TRPM8 is a multimodal sensor of innocuous-to-noxious cold that is activated by several factors, such as temperature, cooling agents (e.g., menthol and icilin), voltage, pressure, and osmolality. TRPM8 is a non-selective cation channel permeable to both monovalent and divalent cations that is activated by multiple factors, such as temperature, voltage, pressure, and changes in osmolality. TRPM8 has attracted great interest because of the therapeutic applications of its modulators that can be utilized for several pathological conditions, including neuropathic pain, irritable bowel syndrome, oropharyngeal dysphagia, chronic cough, and hypertension. At 2.7 Å resolution, it is one of the two highest-resolution structures of any TRPM8 protein that is currently available. Overall, human TRPM8 adopts a characteristic homotetrameric arrangement and is very similar to previously described TRPM8 structures.

We determined a cryo-EM structure of apo HsTRPM8 that was solubilized with lauryl maltose neopentyl glycol (LMNG) and cholesteryl hemisuccinate (CHS). By combining a high-resolution global map with focused refinement maps of N-terminal domains, we were able to build an atomic model of human TRPM8 (HsTRPM8) that comprises residues 43–1104. The pore is composed of helices S5 and S6 connected with a pore helix (PH). The lower gate of the channel is formed by hydrophobic side chains of M978 and F979 (both shown in Fig. 2a as sticks) that close the pore. In contrast, in our reconstruction, only the first two amino acids from the selectivity filter (F912 and G913) are resolved. The conformation of the pore in our structure is similar to the closed C0 MmTRPM812. In our structure, the S4-S5 linker is parallel to the S5 helix, and the S4 helix is fully α-helical. The quality of our EM map in this region allowed us to unambiguously assign them to two CHS molecules and a phospholipid with one monounsaturated fatty acid which we modeled as phosphatidylcholine (POPC). In summary, additional densities visible in our HsTRPM8 (and other published structures) can be interpreted as compounds copurifying with the protein (PE/POPC, Na+) or used for its solubilization (CHS), but we cannot be sure about their identity and source, and thus interpret their physiological relevance. Importantly, we did not observe any density in the putative Ca2+-binding pocket between the S2 and S3 helices that could be assigned to the divalent ion, which further confirms that our structure is not in the desensitized state. To improve the quality of the reconstruction of this region we performed its focused refinement, followed by C4 symmetry expansion and subtraction of the signal from the rest of the TRPM8 molecule.

>[4x]SNSFRAARLSMRNRRNDTLDSTRTLYSSASRSTDLSYSESDLVNFIQANFKKRECVFFTKDSKATENVCKCGYAQSQHMEGTQINQSEKWNYKKHTKEFPTDAFGDIQFETLGKKGKYIRLSCDTDAEILYELLTQHWHLKTPNLVISVTGGAKNFALKPRMRKIFSRLIYIAQSKGAWILTGGTHYGLMKYIGEVVRDNTISRSSEENIVAIGIAAWGMVSNRDTLIRNCDAEGYFLAQYLMDDFTRDPLYILDNNHTHLLLVDNGCHGHPTVEAKLRNQLEKYISERTIQDSNYGGKIPIVCFAQGGGKETLKAINTSIKNKIPCVVVEGSGQIADVIASLVEVEDALTSSAVKEKLVRFLPRTVSRLPEEETESWIKWLKEILECSHLLTVIKMEEAGDEIVSNAISYALYKAFSTSEQDKDNWNGQLKLLLEWNQLDLANDEIFTNDRRWESADLQEVMFTALIKDRPKFVRLFLENGLNLRKFLTHDVLTELFSNHFSTLVYRNLQIAKNSYNDALLTFVWKLVANFRRGFRKEDRNGRDEMDIELHDVSPITRHPLQALFIWAILQNKKELSKVIWEQTRGCTLAALGASKLLKTLAKVKNDINAAGESEELANEYETRAVELFTECYSSDEDLAEQLLVYSCEAWGGSNCLELAVEATDQHFIAQPGVQNFLSKQWYGEISRDTKNWKIILCLFIIPLVGCGFVSFRKKPVDKHKKLLWYYVAFFTSPFVVFSWNVVFYIAFLLLFAYVLLMDFHSVPHPPELVLYSLVFVLFCDEVRQWYVNGVNYFTDLWNVMDTLGLFYFIAGIVFRLHSSNKSSLYSGRVIFCLDYIIFTLRLIHIFTVSRNLGPKIIMLQRMLIDVFFFLFLFAVWMVAFGVARQGILRQNEQRWRWIFRSVIYEPYLAMFGQVPSDVDGTTYDFAHCTFTGNESKPLCVELDEHNLPRFPEWITIPLVCIYMLSTNILLVNLLVAMFGYTVGTVQENNDQVWKFQRYFLVQEYCSRLNIPFPFIVFAYFYMVVKKCFKCCCKEKNMESSVCCFKNEDNETLAWEGVMKENYLVKINTKANDTSEEMRHRFRQLDTKLNDLKGLLKEIANKIK N-(phenylacetyl)glycyl-N~6~-acetyl-L-lysine 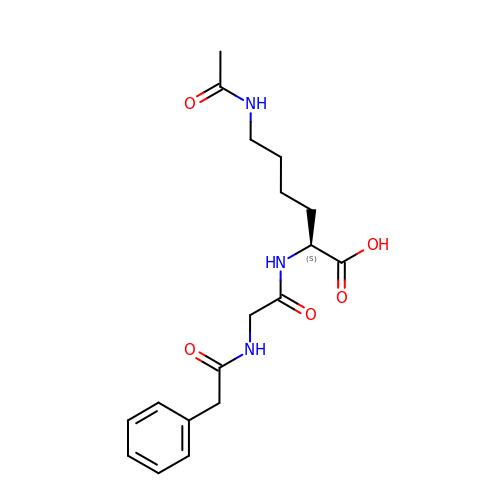| C18 H25 N3 O5 | VCECDMBCQWWZKG-HNNXBMFYSA-N>[5x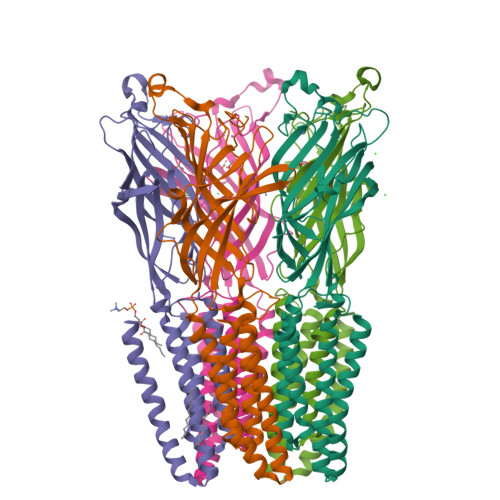]GQDMVSPPPPIADEPLTVNTGIYLIECYSLDDKAETFKVNAFLSLSWKDRRLAFDPVRSGVRVKTYEPEAIWIPEIRFVNVENARDADVVDISVSPDGTVQYLERFSARVLSPLDFRRYPFDSQTLHIYLIVRSVDTRNIVLAVDLEKVGKNDDVFLTGWDIESFTAVVKPANFALEDRLASKLDYQLRISRQYFSYIPNIILPMLFILFISWTAFWSTSYEANVTLVVSTLIAHIAFNILVETNLPKTPYMTYTGAIIFMIYLFYFVAVIEVTVQHYLKVESQPARAASITRASRIAFPVVFLLANIILAFLFFGF> MCKDKNEKKNYEHVNANEKNGYLASEKNELTKNKVEEHTYDYDYVVIGGGPGGMASAKEAAAHGARVLLFDYVKPSSQGTKWGIGGTCVNVGCVPKKLMHYAGHMGSIFKLDSKAYGWKFDNLKHDWKKLVTTVQSHIRSLNFSYMTGLRSSKVKYINGLAKLKDKNTVSYYLKGDLSKEETVTGKYILIATGCRPHIPDDVEGAKELSITSDDIFSLKKDPGKTLVVGASYVALECSGFLNSLGYDVTVAVRSIVLRGFDQQCAVKVKLYMEEQGVMFKNGILPKKLTKMDDKILVEFSDKTSELYDTVLYAIGRKGDIDGLNLESLNMNVNKSNNKIIADHLSCTNIPSIFAVGDVAENVPELAPVAIKAGEILARRLFKDSDEIMDYSYIPTSIYTPIEYGAC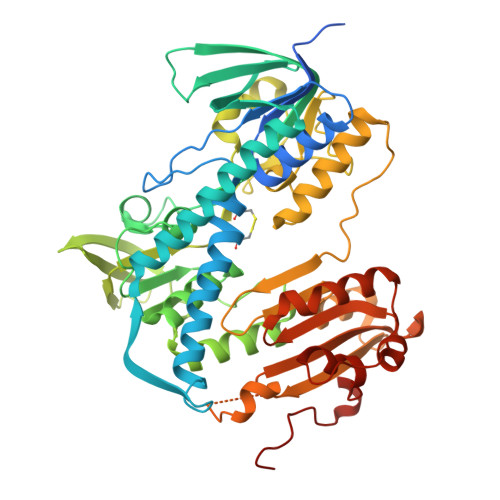GYSEEKAYELYGKSNVEVFLQEFNNLEISAVHRQKHIRAQKDEYDLDVSSTCLAKLVCLKNEDNRVIGFHYVGPNAGEVTQGMALALRLKVKKKDFDNCIGIHPTDAESFMNLFVTISSGLSYAAKGGCGGGKSG>[4x]SNAMKTVTVRDLVVGEGAPKIIVSLMGKTITDVKSEALAYREADFDILEWRVDHFANVTTAESVLEAAGAIREIITDKPLLFTFRSAKEGGEQALTTGQYIDLNRA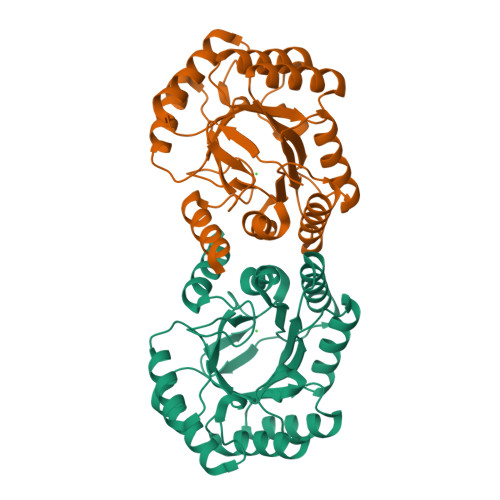AVDSGLVDMIDLELFTGDDEVKATVGYAHQHNVAVIMSNHDFHKTPAAEEIVQRLRKMQELGADIPKIAVMPQTKADVLTLLTATVEMQERYADRPIITMSMSKTGVISRLAGEVFGSAATFGAVKKASAPGQISVADLRTVLTILHQA>MKHTLPDLPFDYADLEPVISHEIMQLHHQKHHATYVNNLNQIEEKLHEAVSKGNLKEAIALQPALKFNGGGHINHSIFWTNLAKDGGEPSKELMDTIKRDFGSLDNLQKRLSDITIAVQGSGWGWLGYCKKDKILKIATCANQDPLEGMVPLFGIDVWEHAYYLQY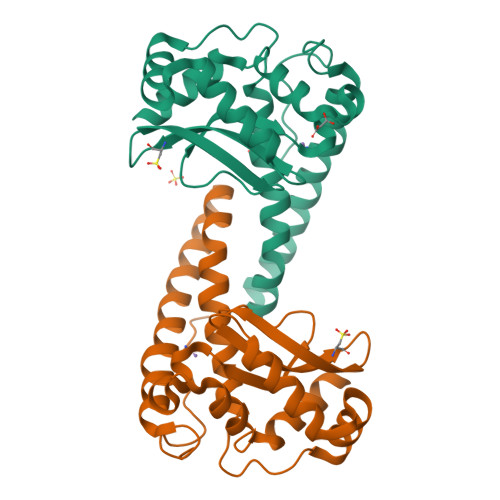KNVRPDYVHAIWKIANWKNISERFANARQ[2x]> GAMVSRRKILSRSRDDLNLDQTFTQQEEEEDIWFQKDKLYKEHIQEVLDKWTQIDD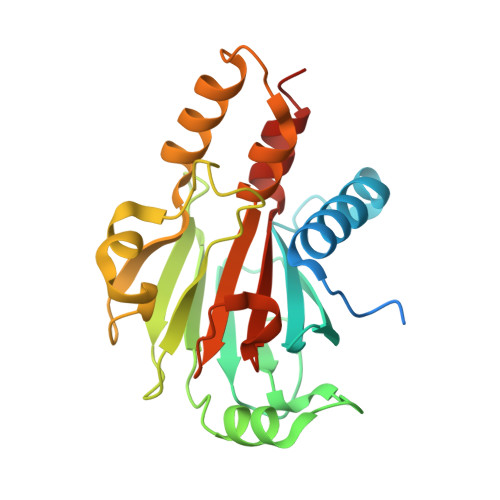EIWAKVIVFERNRRVAKAYARAPVLTINGSDDGFDGMRIGLCGFDNPMRDQKTDEMKRVIGQGVKIKMDDAGNILIRRYAKSNVYVKSTASSPNEETSIGAEILKLPNQALESEKIVKLFDMKKFQSNVNRELRRAYPDRRRLETQCLSAVAFVKSENDILECPIWVLIVNVVAMDMLKSKLPPVQ> GSPALDTGTTEEDRLKIDVIDWLVFDPAQRAEALKQGNAIMRKFLASKKHEAAKEVFVKIPQDSIAEIYNQCEEQGMESPLPAEDDNAIREHLCIRAYLEAHETFNEWFKHMNSVPGGSGGSWKGHLDALTADVKEKMYNVLLFVDGGWMVDVREDAKEDHERTHQMVLLRKLCLPMLCFLLHTILHSTGQYQECLQLADMVSSERHKLYLVFSKEELRKLLQKLRESSLMLLDQGLDPLGYEIQL;> MASHHLSWLHEINSQELEKAHATLLGLANMETRYFAKKKTLLGLSKLAALASDFSEDMLQEKIEEMAEQERFLLHQETLPEQLLAEKQLNLSAMPVLTAPQL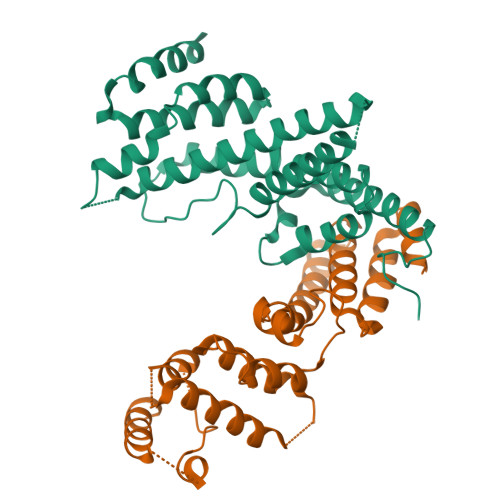IGLYICEENRRANEYDFKKALDLLEYIDEEEDININDLKLEILCKALQRDNWSSSDGKDDPIEVSKDSIFVKILQKLLKDGIQLSEYLPEVKDLLQADQLGSLKSNPYFEFVLKANYEYYVQGQI>VSHQQGQSHLFECDYPISADTYVINWYKDGTSVMNYLSGGEPAFTEDLDDRTDVQFVNNRNLEITNLRVSDEGEYYCSVIE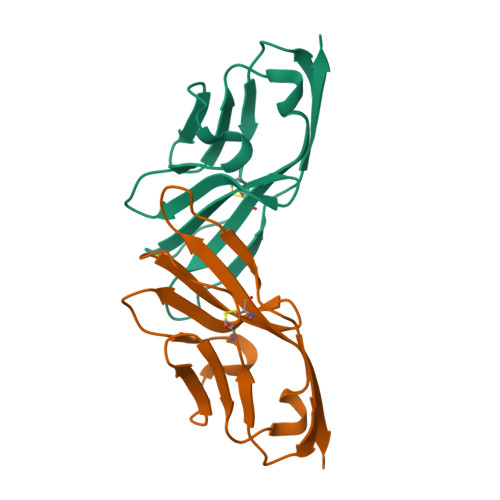IGAGGQSGDGTRYQLVVFV[2x]>MEELKKIAGVRAAQYVEDGMIVGLGTGSTAYYFVEEVGRRVQEEGLQVIGVTTSSRTTAQAQALGIPLKSIDEVDSVDVTVDGADEVDPNFNGIKGGGGALLMEKIVGTLTKDYIWVVDESKMVDTLGAFRLPVEVVQYGAERLFREFEKKGYKPSFREYDGVRFVTDMKNFIIDLDLGSIPDPIAFGNMLDHQVGVVEHGLFNG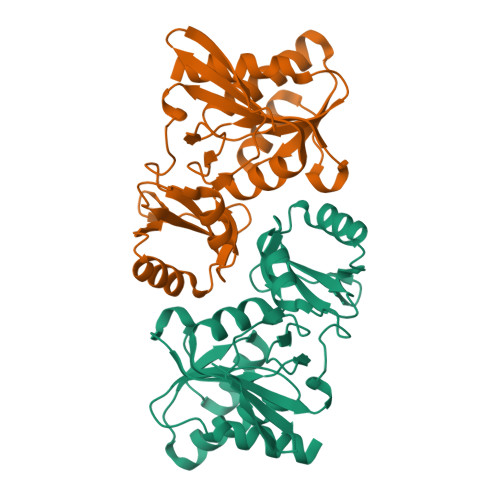MVNRVIVAGKDGVRILEANK[2x]>MRGSHHHHHHGSMDKNIIIGAMTALITPFKNGKVDEQSYARLIKRQIENGIDAVVPVGTTGESATLTHEEHRTCIEIAVETCKGTKVKVLAGAGSNATHEAVGLAKFAKEHGADGILSVAPYYNKPTQQGLYEHYKAIAQSVDIPVLLYNVPGRTGCEISTDTIIKLFRD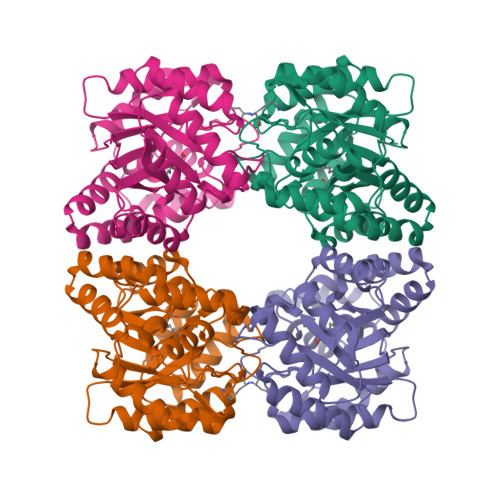CENIYGVKEASGNIDKCVDLLAHEPRMMLISGEDAINYPILSNGGKGVISVTSNLLPDMISALTHFALDENYKEAKKINDELYNINKILFCESNPIPIKTAMYLAGLIESLEFRLPLCSPSKENFAKIEEVMKKYKIKGF[12x]> GHMIDRRRGLGRRRKSWAKSHGFDYEYESEDLLKRWKRGVMSTVGDVTAKNVVLGQIRGEAVFIFDIEEV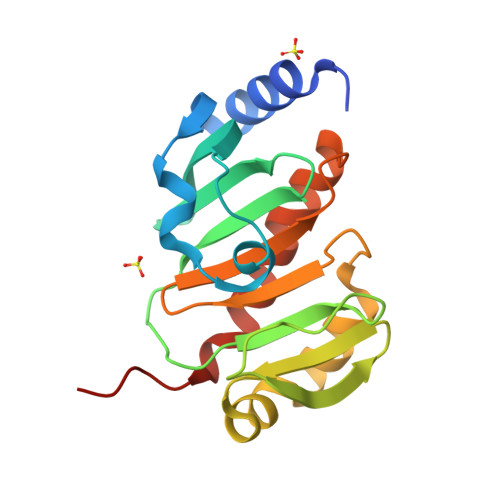ATVIALHRKVGTNVVVDLRLKGLKEPRENDIWLLGAIGPRMVYSTNLDAARRACDRRMVTFAHTAPDCAEIMWNEQNWTLVAMPVTSNRAQWDEGLRTVRQFNDLLRVLPPVPQNAS> GTSSMADIGSTNDALDYYLKSKGFNGLFSQIELSFSASNLRDRDVLSKSDPMVVVYQKEKDATLSEVFRSEVVLNSLAPKWIKKFIVAYHFETVQTLVFRVYDVDTKFQNSREEMLKLDEQQFLGEATCALSEIITKSTRTSTLELKRKDGFAPQAQPHHGKLIIHAEESLASKISTEIVFRCSNLESKDLFSKSDPFLVVSKIVEHGT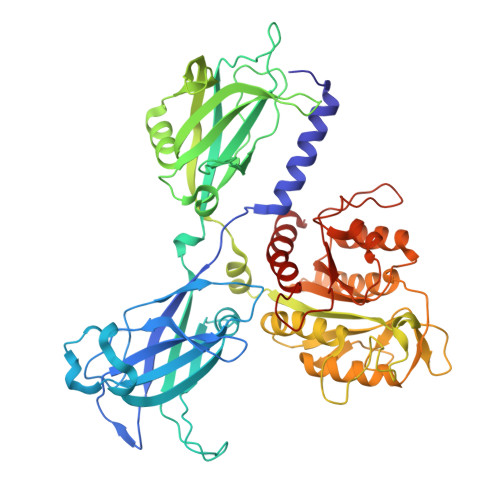PIPVSKTEVRKNDLNPIWKPVFLSVQQVGSKDSPVIIECSDFNSNGKHSLIGKVQKSLSDLEKLHLAGQGINFSLPTGAGQNKVLKSQLFVDKFTETVHHTFLEYLASGFELNFMVAIDFTASNGNPRLPDSLHYIDPSGRLNAYQRAIMDVGEVLQFYDSDKRFPAWGFGARPIDAPVSHCFNLNGSSSYSEVDGIQGIMTSYTSALFNVSLAGPTLFGPVINAAAMIASASLAQGSRKYYVLLIITDGVITDLQETKDALVSASDLPLSILIVGVGGADFKEMEILDADKGERLESSSGRLASRDIVQFVALRDVQYGEISVVQALLAELPSQFLTYMRIRN> MGSSHHHHHHSQDPMDIKINGIKKYTIHVLAKVSASGMEFTQEKDFEHQLLLTDMLETVIRKSVEVNPVLHFHLRKSIIMNHSYFILGLNYIPPAFATKNVKSIHEIYQAIQDVNDLQLLDEFEKSKEKLINKIQQYKHSDSHSGSIRLKDRLFADKKYGSDRLGNFEKMNKITDNIIYAAPDMVNKICEGDGLFYHINDGAIHISNIKDFNYYIPAVINEGVEDIRTDFSKEYSILTCAYTFEHVTDLEREILIPMFDGYIGKYGHSVLFKTLRLVDENLYHISSHYDQESNLLFITVLCSKNQLSTILTKIQHTIESIEFDSVSFSLSKVMFENESRFRFE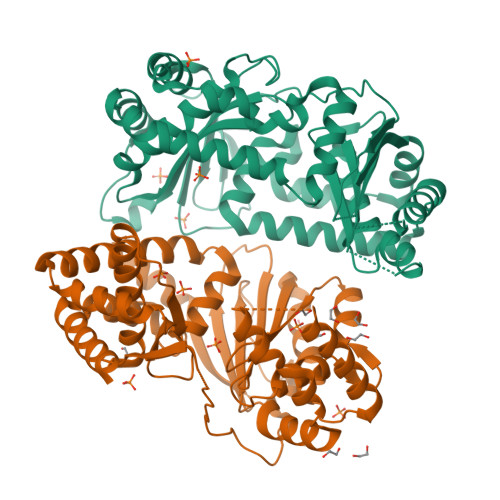DINGLLSHVIKQHGEYKNPESFLKAIQNTDIADFYRLKANMRWVGTSIVEGG;> MLNKSFVKKLDESLNRKQVGSTNVTRYKIEDSYLVLAAVRVGIGGLTYHNGAAHFLEHLKFWRYGENIYNLFFQRGAILNAYTTLEFTDYVFLSKEESINENLNLLLTFLYHHQYDEKTISLERNIIINEINGAGTARLNGQESIEKERHCILGSAESISRMGRKEFELISQKYYTPENTSIYVIGGNQDIDLFHIPTAVMTTQYGKPTHKVNVNEVEMNKDMILLPVEHGDYLKNRMICHLIADMIKHLAQQLEYDVSVGLFISTNQHSCYLKVKKSDQKRFSSLIQQLSMDEHFIETYIKDYQWRFMNELVINFNQLHNIYDYMTEYRLGEYTVAELFGSLDSVDKLDILAVRNELINQLTVGE>[2x]MATLTAKNLAKAYKGRRVVEDVSLTVNSGEIVGLLGPNGAGKTTTFYMVVGIV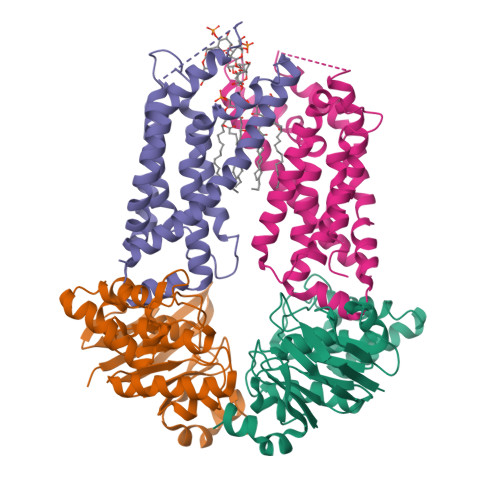PRDAGNIIIDDEDISLLPLHARARRGIGYLPQEASIFRRLSVYDNLMAVLQIRDDLTSEQREDRAKELMEEFHIEHLRDSLGQALSGGERRRVEIARALAANPKFILLDEPFAGVDPISVIDIKRIIEHLRDSGLGVLITDHNVRETLAVCERAYIVSQGHLIAHGTPQQILEDEQVKRVYLGEDFRL;> MIIIRYLVRETLKSQLAILFILLLIFFCQKLVRILGAAVDGDIPTNLVLSLLGLGIPEMAQLILPLSLFLGLLMTLGKLYTESEITVMHACGLSKAVLIKAAMILALFTGAVAAVNVMWAGPWSSRHQDEVLAEAKANPGMAALAQGQFQQASDGNAVMFIESVNGNRFHDVFLAQLRPKGNARPSVVVADSGELSQQKDGSQVVTLNKGTRFEGTAMLRDFRITDFNNYQAIIGHQAVSADPDDTEQMDMRTLWKTHTDRARAELHWRFTLVATVFIMALMVVPLSVVNPRQGRVLSMLPAMLLYLVFFLLQTSIKSNGGKGKMDPAIWMWAINLLYFALAVLLNLWDTVPMRRFRARFNKGAA;> MQAFGVLDRYIGKTIFNTIMMTLFMLVSLSGIIKFVDQLKKSGQGSYDALGAGLYTILSVPKDIQIFFPMAALLGALLGLGMLAQRSELVVMQASGFTRLQVALAVMKTAIPLVLLTMAIGEWVAPQGEQMARNYRAQQMYGGSLLSTQQGLWAKDGHNFVYIERVKGNDELGGVSIYAFNPERRLQSVRYAASAKFDSENKVWRLSQVDESDLTDPKQVTGSQMVSGTWKTNLTPDKLGVVALDPDALSISGLHNYVKYLKSSGQDPGRYQLNMWSKIFQPLSVAVMMLMALSFIFGPLRSVPMGVRVVTGISFGFIFYVLDQIFGPLTLVYGIPPIIGALLPSASFFLISLWLMMRKA1-(3,4-difluorobenzyl)-2-oxo-N-{(1R)-2-[(2-oxo-2,3-dihydro-1H-benzimidazol-5-yl)oxy]-1-phenylethyl}-1,2-dihydropyridine-3-carboxamide 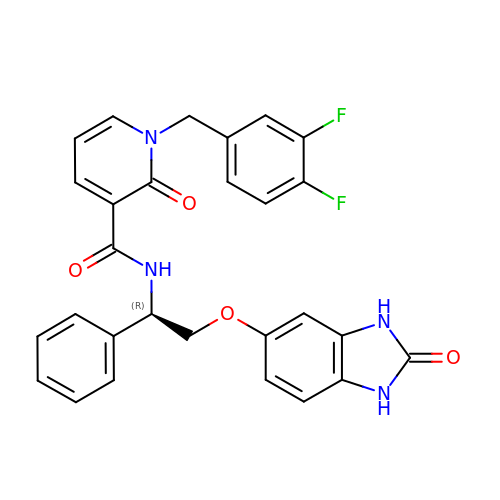| C28 H22 F2 N4 O4 | GCWCGSPBENFEPE-VWLOTQADSA-N>YKWHYSGLNRWHGAGSTADFQKIIQERCDTYTQTIRPGSRSRNCQAIRQAFMSAFISKDPCKATKEDYNSLINLAPPTVPCGQQVFWSKTKELAHEYAKRRRLMTLEDTLLGYLADGLRWCGEPGSSDLNIWSCPDWRKDCRTNYLSVFWEVLSERFAESACNTVRVVLNGSLENAFDSMSIFGRVEAPNLRPQVELEAWLVHDTGKPPSDSCSGSSIRKLKSILDGRNVKFRCMDNLSRDQFLQRS[2x]

Altogether CD38 appears to be a key player in the biosynthesis of calcium messengers which are involved in a wide range of cellular functions. Thus, the catalytic transformation of NAD+ involves the formation, via a ribooxocarbenium ion-like transition state, of a unique reaction intermediate that partitions between several competing pathways such as an irreversible hydrolytic process leading to ADP-ribose and a reversible minor pathway that governs the formation of cADPR. The L-shaped structure of bCD38 consists of two distinct domains separated by a cleft and connected by a hinge region. α-Helices are found mainly in the N-terminal and membrane-proximal domain of this transmembrane protein, whereas β-sheets are preponderant in the distal C-terminal domain. The active site of bCD38 consists in a funnel-shaped cavity with a fairly rigid structure; it buries the NMN+ moiety of the substrate and its scissile bond in its deepest non-polar and least solvent accessible region, whereas the AMP moiety interacts with its more solvent-exposed region, at the entrance of the catalytic cleft.

The active site of bCD38 consists in the largest solvent accessible cavity detected at the surface of the protein. A cluster of three strictly conserved phenylalanine residues (Phe117, Phe188 and Phe214) acts as a hydrophobic ‘plug’, sealing the bottom of this pocket. In the unliganded state, Glu218 is also stabilized by water molecules, e.g. two molecules bridge via hydrogen bonds its Oε1 and Oε2 atoms with the backbone amide group of Trp118. Several other water molecules are present in this region of the active site of apo wt bCD38; four of them are in line and hydrogen bonded to the backbone of the first β-strand of bCD38 C-ter domain between residues Val116 and Lys120. This cluster of water molecules could provide a means of access for bulk water to the bottom of the active site. In apo bCD38, the residues of the ‘signature motif’, despite being solvent-exposed, have also a limited conformational flexibility. This is mainly due to the occurrence of an extensive hydrogen bond system that also involves water molecules.> GGCUUAUCAAGAGAGGGA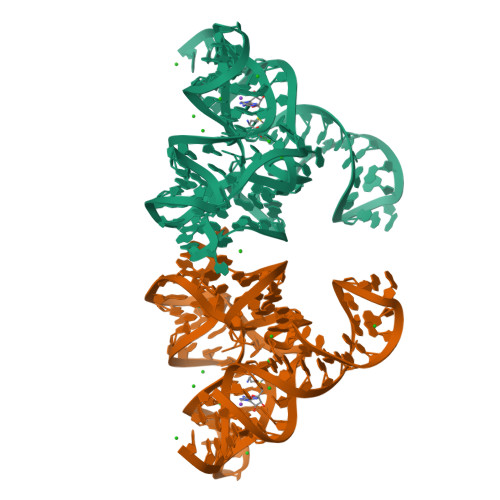GAGCGACUGGCGCGAAGAUCCCCGGCAACCAGAAAUGGUGCCAAUUCCUGCAGCGGAAACGUUGAAAGAUGAGCCG> CDDNTGGLGLGMFPGNDQNIKGKLSTFDVTTESVKTGDIYAKTNIGYIGKFTDETFGTYQAGFLAQLNCPDGLTFPEPYKEVTDASGNVISATGRMVVDDKDPENKDVTFIKDGNQIIGNIRAVELYLWYDSYFGDSLTACRLSVYELGGNGKETLNLDNAYYTDINPEDFYDSQNILGTKAYTAVDLSVKDSIRNLSTYVPSVHIAFKEDIATRVGGNILTAARKAKNADKEFNSQLFREAFQGIYVKSDYGDGTVLYIDQPQMNVVYKCYATDSITGKKLQKKDGSGKDSTYYSYRVFATTREVIQANQLKNDPERIDALIKEDKNTYLKSPAGIFTEATLPISDIQNELTGDTLNAVKLTFTNYNQTGDKKFGMAIPSTVMLVRKKFQDSFFKDNKLSDGVSSYLTSHTSSTNQYVFSNITKLVNACIAEKEEAKKNAGSSWDETKWLQENPDWNKVVLIPVLVTYDSSNTTTGQANIIRIQHDLKPGYVRLKGGSLGKTNPDYKLKLEVISTDFGLTTKSN;> MRIKFLSIIASFFMVSFVITSCLDNDNEVNYSPDATIRAFELDTIGYGVNYKFTIDQVSRLIYNVDSLPVNADTIINSILIKTLTTASGIVTMKDQNDQDSIVNINDSIDLTKYVNATEKNNFLVLKVWAPNMEVQNEYKVNIRMHTMVPDSLSWGKDPIANNPVRNTAEKQKVVTLGDKILLFAQNNEIYSTAIPAGSPTDRLNYGQKWDKETTGKLPDGADVTSIIRFVDKLYLLTKNKEVYNSNDGLTWTKDEVLNSDGVSVTNLITSFSDSDGSNHKKINGIAGIVEINGEKYFSFAEKDVTWEKDIDKLTVVPAEFPINNLSADVYATESGTLNAIVVGNTEDGLDNDTATVVWASEDGKAWIPMEIPSNNNCPKLVDPSIIHYNDAFYICGKETKDDAKGFQKFYTSPTLLVWKGVDRMFMLPGILPPVKLEGGVTQHPSLHESSFKGKEVNYTMVVDRNHYIWMVGGQGIDKIWRGRVNKLGFLIQ;> MSKKIYLFSLVLLALAFVSCSETEEVGKYDNWRARNEAFIDSLANVYATASGRGGLERIEMLTAPGNYIYYKEMEPMTDHVVKAGNPKYTDYVKVYYKGTNILGEYFDGNFKGDNPVVDGKDPSEGDSPTTIFQVSGVITGWGEVLQRMEVGDRWKVYIPWDYAYGSSGTTGILGYSALVFDITLLDFANTEAELK;> MKKLVFLFLSLLAAGGIFQACDDSKTYAEMLEDEKNAVNKFIKDKGIRIISQDEFEKNDTVTNLERNEYVALSDGVYMQIVDRGSAENKTDTFANNNEICVRYIEEDIMTRDTTCFNVFLEEWGDANQLYTNPAVFRYVAEGSYVYGTFIQMDYYWASYYQSTAVPAGWLLALPFVRNYAHVRLIVPSKVGHSSAQQYVNPYYYDIWTFSKALN

The β-barrel assembly machinery (BAM) complex is a conserved, multiprotein machine that mediates the folding and membrane insertion of newly synthesized β-barrel outer membrane (OM) proteins. Cryogenic electron microscopy (cryo-EM) structures of the BAM complexes from the gut commensal B. thetaiotaomicron and the oral pathogen Porphyromonas gingivalis are similar and reveal a 7-protein, ~325-kDa complex with most of its mass on the extracellular side. Remarkably, besides BamA and BamD subunits, Bacteroidetal BAM contains a 14-stranded integral OMP that is intimately associated with BamA. The remaining four components, named BamH–K, are all SLPs and form an extracellular dome-like structure over BamA that may provide additional functionality to enable the folding and assembly of the many β-barrel–SLP complexes that are a hallmark of the Bacteroidota.

Class 1 lacks density for the periplasmic components but has good density for all extracellular proteins, whereas class 2 has modest resolution for BamA POTRA domains 4 and 5 and for part of BamD, but with poorly resolved extracellular areas. The crescent-shaped BamH subunit is positioned over the BamA barrel and forms an arch-like structure approximately 60 Å above the OM surface. BamH interacts with BamI and BamJ on one side and with BamK on the other. Based on its structure and the conservation of the protein core, BamH probably functions as a scaffold. The highly conserved N-terminus of BamH is wedged between two strands of the BamG barrel and interacts with the conserved BamG N-terminus, and the tri-acylated BamH lipid anchor is positioned at the BamAG interface. Of the remaining three components, BamI consists of two domains. The small N-terminal domain is conserved and interacts with the BamJ PPI, whereas the less-conserved C-terminal domain contacts BamH and adopts a six-bladed β-propeller fold, with each blade consisting of three to four β-strands. The conservation analysis of both BamJ and BamK indicates that their putative active sites are directed towards the interior of the BAM dome. BamH–K all have glycosylation sites, with by far the most present on BamI.>[2x]GSTPDYLMQLMNDK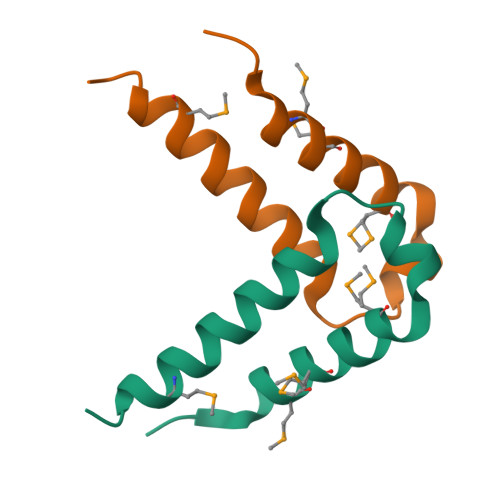KLMSSLPNFSGIFNHLERLLDEEISRVRKDMYNDTLNGSTEK>VVGGTEAQRNSWPSQISLQYRSGSSWAHTCGGTLIRQNWVMTAAHCVDRELTFRVVVGEHNLNQNDGTEQYVGVQKIVVHPYWNTDDVAAGYDIALLRLAQSVTLNSYVQLGVLPRAGTILANNSPCYITGW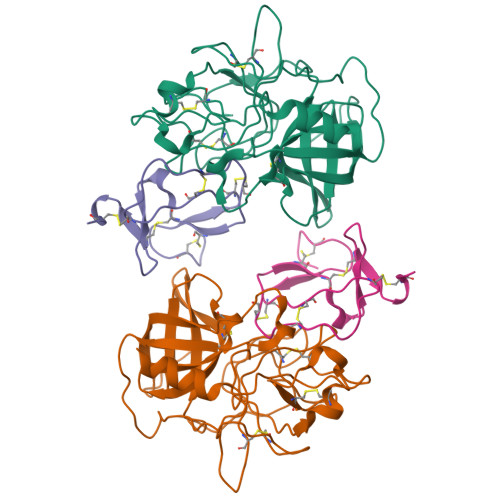GLTRTNGQLAQTLQQAYLPTVDYAICSSSSYWGSTVKNSMVCAGGDGVRSGCQGDSGGPLHCLVNGQYAVHGVTSFVSRLGCNVTRKPTVFTRVSAYISWINNVIASN[2x];>[2x]GQESCGPNEVWTECTGCEMKCGPDENTPCPLMCRRPSCECSPGRGMRRTNDGKCIPASQCP4-NITROPHENYL PHOSPHATE | C6 H6 N 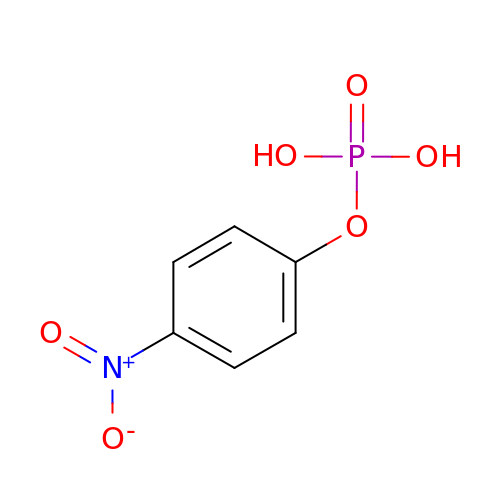O6 P | XZKIHKMTEMTJQX-UHFFFAOYSA-N>MSLPETKSDDILLDAWDFQGRPADRSKTGGWASAAMILCIEAVERLTTLGIGVNLVTYLTGTMHLGNATAANTVTNFLGTSFMLCLLGGFIADTFLGRYLTIAIFAAIQATGVSILTLSTIIPGLRPPRCNPTTSSHCEQASGIQLTVLYLALYLTALGTGGVKASVSGFGSDQFDETEPKERSKMTYFFNRFFFCINVGSLLAVTVLVYVQDDVGRKWGYGICAFAIVLALSVFLAGTNRYRFKKLIGSPMTQVAAVIVAAWRNRKLELPADPSYLYDVDDIIAAEGSMKGKQKLPHTEQFRSLDKAAIRDQEAGVTSNVFNKWTLSTLTDVEEVKQIVRMLPIWATCILFWTVHAQLTTLSVAQSETLDRSIGSFEIPPASMAVFYVGGLLLTTAVYDRVAIRLCKKLFNYPHGLRPLQRIGLGLFFGSMAMAVAALVELKRLRTAHAHGPTVKTLPLGFYLLIPQYLIVGIGEALIYTGQLDFFLRECPKGMKGMSTGLLLSTLALGFFFSSVLVT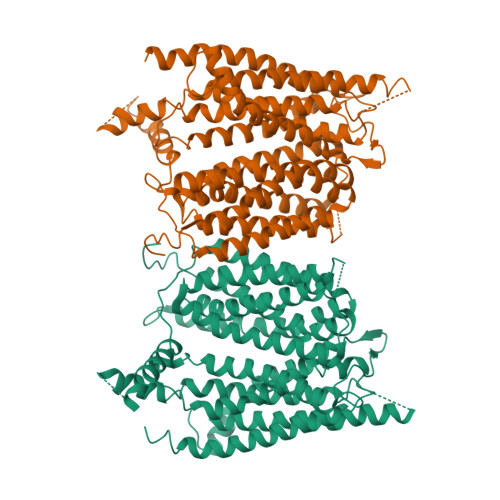IVEKFTGKAHPWIADDLNKGRLYNFYWLVAVLVALNFLIFLVFSKWYVYKEKRLAEVGIELDDEPSIPMGH[2x]>[2x]DHPFTEIKSGFLERRSKFLKSYSKGYYVL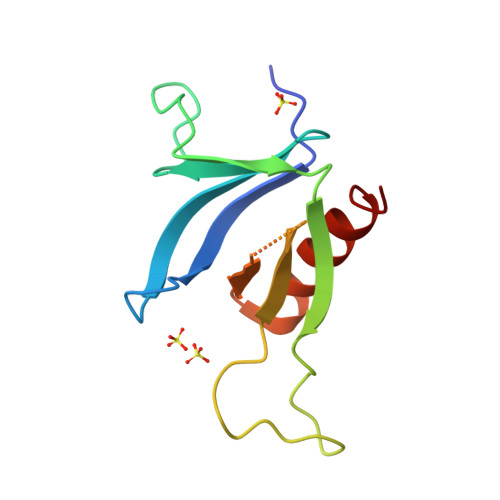TPNFLHEFKTADRKKDLVPVMSLALSECTVTEHSRKNSTSSPNSTGSDAKFVLHAKQNGIIRRGHNWVFKADSYESMMSWFDNLKILTSTS>MLVVPAIDLFRGKVARMIKGRKENTIFYEKDPVELVEKLIEEGFTLIHVVDLSNAIENSGENLPVLEKLSEFAEYIQIGGGIRSLDYAEKLRKLGYRRQIVSSKVLEDPSSLKSLREIDVEPVFSLVTRGGRVAFKGWLAEEEIDPVS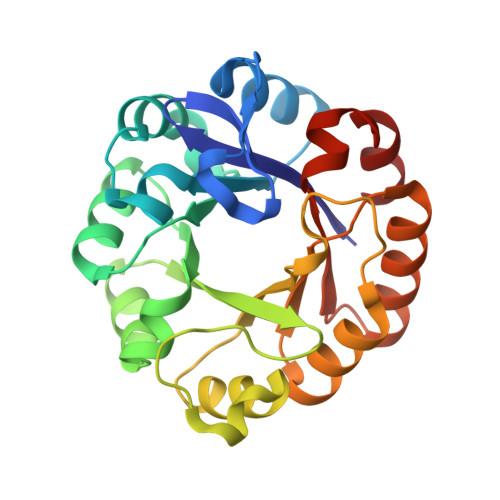LLKRLKEYGLEEIVHTEIEKVGTLQEHDFSLTKKIAIEAEVKVLAAGGISSENSLKTAQKVHTETNGLLKGVIVGRAFLEGILTVEVMKRYAR[2x]>MSLSPSARRVQGALETRGFGHLKVVELPASTRTAKEAAQAVGAEVGQIVKSLVFVGEKGAYLFLVSGKNRLDLGKATRLVGGPLRQATPEEVRELTGFAIGGVPPVGHNTPLPAYLDEDLLGYPEVWAAGGTPRALFRATPKELLALTGAQ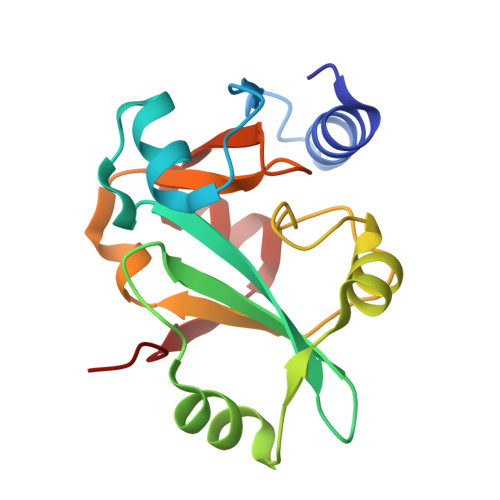VADLKEG[4x]>[3x]KETAAAKFERQHMDSGGGGSGHMENGYTYEDYKNTAEWLLSHTKHRPQVAIICGSGLGGLTDKLTQAQIFDYGEIPNFPRSTVPG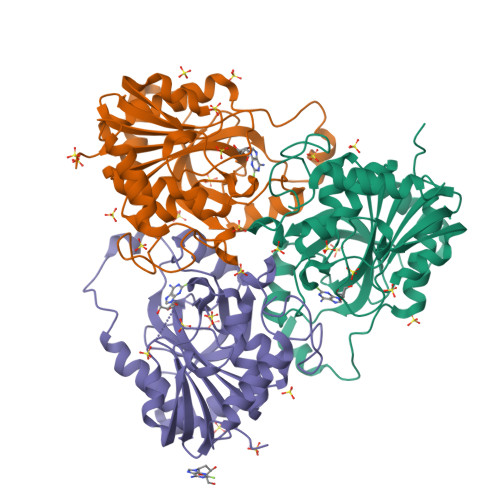HAGRLVFGFLNGRACVMMQGRFHMYEGYPLWKVTFPVRVFHLLGVDTLVVTNAAGGLNPKFEVGDIMLIRDHINLPGFSGQNPLRGPNDERFGDRFPAMSDAYDRTMRQRALSTWKQMGEQRELQEGTYVMVAGPSFQTVAECRVLQKLGADAVGMSTVPEVIVARHCGLRVFGFSLITDKVIMDYESLEKANHEEVLAAGKQAAQKLEQFVSILMASIPLPDKAS> HMASMKKKGSVVIVGRINLSGDTAYAQQTRGEEGCQETSQTGRDKNQVEGEVQIVSTATQTFLATSINGVLWTVYHGAGTRTIASPKGPV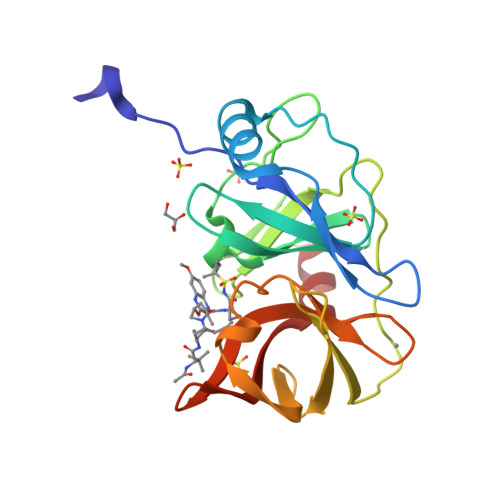TQMYTNVDKDLVGWQAPQGSRSLTPCTCGSSDLYLVTRHADVIPVRRRGDSRGSLLSPRPISYLKGSSGGPLLCPAGHAVGIFRAAVSTRGVAKAVAFIPVESLETTMR>MFHSSAMVNSHRKPMFNIHRGFYCLTAILPQICICSQFSVPSSYHFTEDPGAFPVATNGERFPWQELRLPSVVIPLHYDLFVHPNLTSLDFVASEKIEVLVSNATQFIILHSKDLEITNATLQSEEDSRYMKPGKELKVLSYPAHEQIALLVPEKLTPHLKYYVAMDFQAKLGDGFEGFYKSTYRTLGGETRILAVTDFEPTQARMAFPCFDEPLFKANFSIKIRRESRHIALSNMPKVKTIELEGGLLEDHFETTVKMSTYLVAYIVCDFHSLSGFTSSGVKVSIYASPDKRNQTHYALQASLKLLDFYEKYFDIYYPLSKLDLIAIPDFAPGAMENWGLITYRETSLLFDPKTSSASDKLWVTRVIAHELAHQWFGNLVTMEWWNDIWLKEGFAKYMELIAVNATYPELQFDDYFLNVCFEVITKDSLNSSRPISKPAETPTQIQEMFDEVSYNKGACILNMLKDFLGEEKFQKGIIQYLKKFSYRNAKNDDLWSSLSNSCLESDFTSGGVC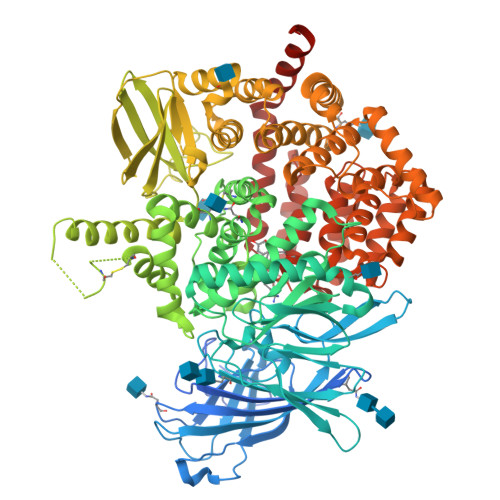HSDPKMTSNMLAFLGENAEVKEMMTTWTLQKGIPLLVVKQDGCSLRLQQERFLQGVFQEDPEWRALQERYLWHIPLTYSTSSSNVIHRHILKSKTDTLDLPEKTSWVKFNVDSNGYYIVHYEGHGWDQLITQLNQNHTLLRPKDRVGLIHDVFQLVGAGRLTLDKALDMTYYLQHETSSPALLEGLSYLESFYHMMDRRNISDISENLKRYLLQYFKPVIDRQSWSDKGSVWDRMLRSALLKLACDLNHAPCIQKAAELFSQWMESSGKLNIPTDVLKIVYSVGAQTTAGWNYLLEQYELSMSSAEQNKILYALSTSKHQEKLLKLIELGMEGKVIKTQNLAALLHAIARRPKGQQLAWDFVRENWTHLLKKFDLGSYDIRMIISGTTAHFSSKDKLQEVKLFFESLEAQGSHLDIFQTVLETITKNIKWLEKNLPTLRTWLMVNTRHHHHHH[2x]2-[1-(3-fluoro-4-hydroxyphenyl)-1H-1,2,3-triazol-4-yl]-7-methyl-1,7-naphthyridin-8(7H)-one 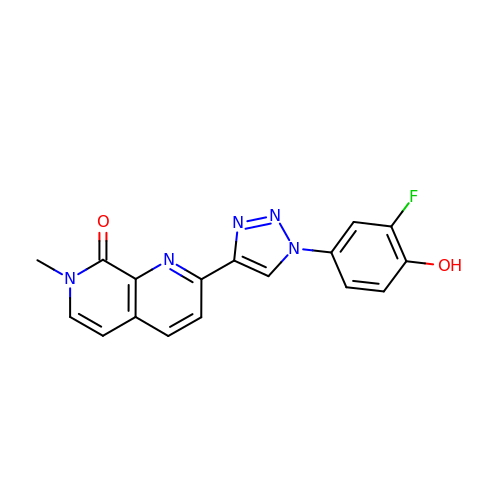| C17 H12 F N5 O2 | VGLQAFZICPSJRO-UHFFFAOYSA-N>ATTHLDVCAVVPAAGFGRRMQTECPKQYLSIGNQTILEHSVHALLAHPRVKRVVIAISPGDSRFAQLPLANHPQITVVDGGDERADSVLTGLKAAGDAQWVLVHDAARPCLH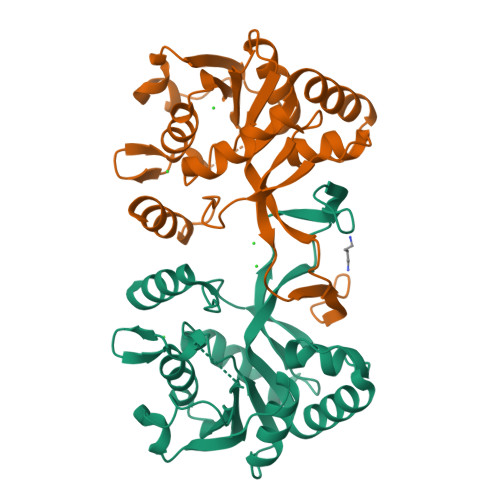QDDLARLLALSETSRTGGILAAPVRDTMKRAEPGKNAIAHTVDRNGLWHALTPQFFPRELLHDCLTRALNEGATITDEASALEYCGFHPQLVEGRADNIKVTRPEDLALAEFYLTRTIHQENT[2x]> APLLLYANRRDLRLVDATNGKENATIVVGGLEDAAAVDFVFSHGLIYWSDVSEEAIKRTEFNKTESVQNVVVSGLLSPDGLACDWLGEKLYWTDSETNRIEVSNLDGSLRKVLFWQELDQPRAIALDPSSGFMYWTDWGEVPKIERAGMDGSSRFIIINSEIYWPNGLTLDYEEQKLYWADAKLNFIHKSNLDGTNRQAVVKGSLPHPFALTLFEDILYWTDWSTHSILACNKYTGEGLREIHSDIFSPMDIHAFSQQRQPNATNPCGIDNGGCSHLCLMSPVKPFYQCACPTGVKLLENGKTCKDGATELLLLARRTDLRRISLDTPDFTDIVLQ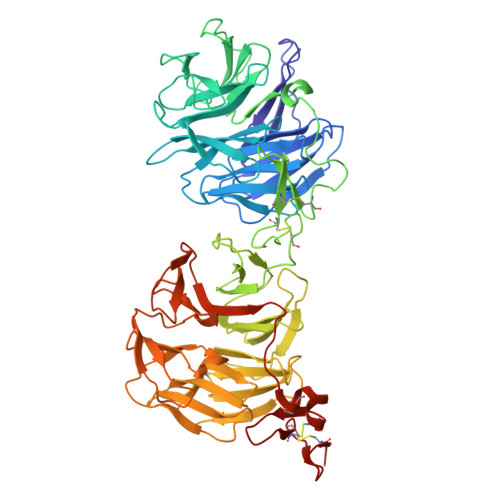LEDIRHAIAIDYDPVEGYIYWTDDEVRAIRRSFIDGSGSQFVVTAQIAHPDGIAVDWVARNLYWTDTGTDRIEVTRLNGTMRKILISEDLEEPRAIVLDPMVGYMYWTDWGEIPKIERAALDGSDRVVLVNTSLGWPNGLALDYDEGKIYWGDAKTDKIEVMNTDGTGRRVLVEDKIPHIFGFTLLGDYVYWTDWQRRSIERVHKRSAEREVIIDQLPDLMGLKATNVHRVIGSNPCAEENGGCSHLCLYRPQGLRCACPIGFELISDMKTCIVP> MIIPALNLIGGTVVRVVRLHQGDYARQRDYGNDPLPRLQDYAAQGAGVLHLVDLTGAKDPAKRQIPLIKTLVAGVNVPVQVGGGVRTEEDVAALLKAGVARVVIGSTAVKSPDVVKGWFERFGAQALVLALDVRIDEHGTKQVAVSGWQENSGVSLEQLVETYLPVGL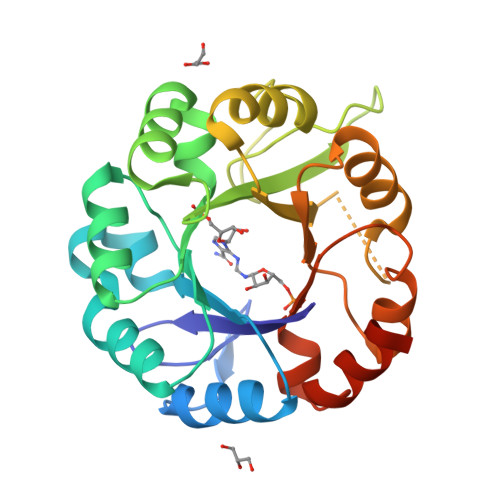KHVLCTDISRDGTLAGSNVSLYEEVCARYPQIAFQSSGGIGDIDDIAALRGTGVRGVIVGRALLEGKFTVKEAIQCWQNVKGHHHHHH>[3x]PLNSPNVYDV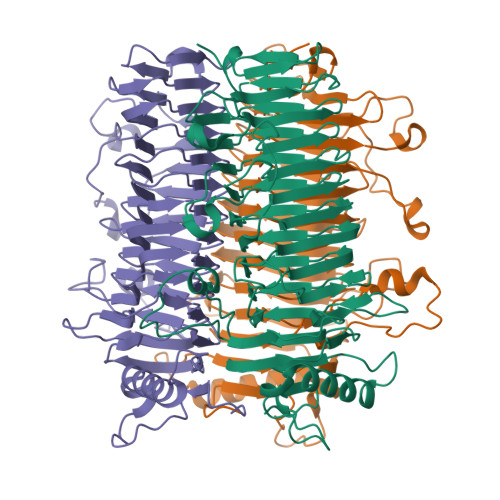TAWRIKGQPKVTAESDIGAVINDIIADIKKRQSTPETRPGAVVIIPPGDYDLHTQVVVDVDYLTIAGFGHGFFSRSIKDNVDTTGWLNLQPGGSHIRVLTPPTSPQAFLVRRDGSPRLSGIVFKDFCLDGVSFVPDGNSYKNGKTGIDVASDNDSIHITGMGFVYLEHALIVRGADALRVHDNMVAECGNCVELTGAGQATIVSDNLMGAGPEGVTLLAENHEGLLVTGNNFFPRGRSLLEFTGCNRCSVTSNRFQGFYPGMMRLLNGCKENLITSNHFRRGTEGFPPFIDRTNGLDDLYGVIHAMGDNNLISNNLFAYDVPPGKIAPAGAQPTIMLIAGGDGNVIATNHVISNVDTQHVVLDGSATRSKVLDSGAASTITSYSPDTAIRPTPH> KETAAAKFERQHMDSSTSAASSSNYCNQMMKSRNLTKDRCKPVNGFVHESLADV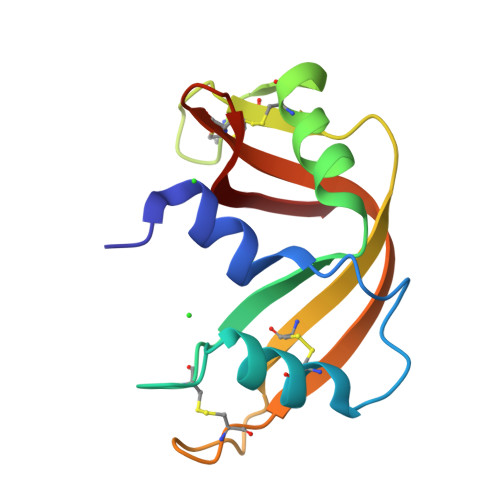QAVCSQKNVACKNGQTNCYQSYSTMSITDCRETGSSKYPNCAYKTTQANKHIIVACEGNPYVPVHFDASV>[2x]GSHMGSKSSAAKEGAGAVDEEDFIKAFDDVPVVQIYSSRDLEESINKIREILSDDKHDWEQRVNALKKIRSLLLAGAAEYDNFFQHLRL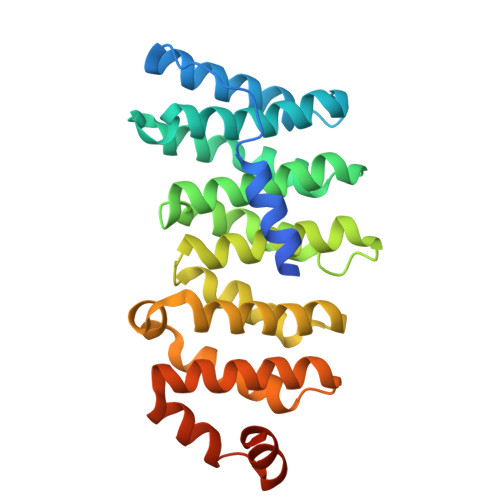LDGAFKLSAKDLRSQVVREACITLGHLSSVLGNKFDHGAEAIMPTIFNLIPNSAKIMATSGVVAVRLIIRHTHIPRLIPVITSNCTSKSVAVRRRCFEFLDLLLQEWQTHSLERHISVLAETIKKGIHDADSEARIEARKCYWGFHSHFSREAEHLYHTLESSYQKALQSHLKNSDSIVSLPQS> MIIKRTPQAASPLASWLSYLENLHSKTIDLGLERVSLVAARLGVLKPAPFVFTVAGTNGKGTTCRTLES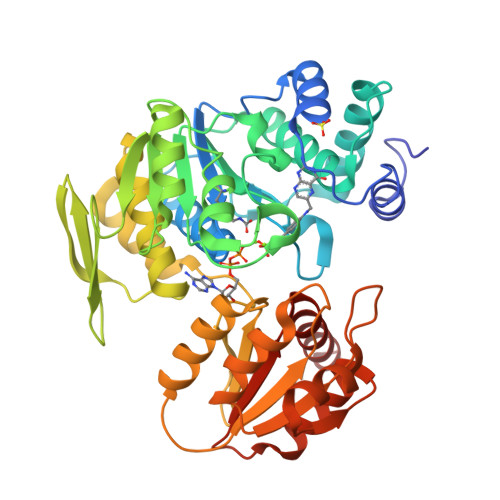ILMAAGYKVGVYSSPHLVRYTERVRVQGQELPESAHTASFAEIESARGDISLTYFEYGTLSALWLFKQAQLDVVILEVGLGGRLDATNIVDADVAVVTSIALDHTDWLGPDRESIGREKAGIFRSEKPAIVGEPEMPSTIADVAQEKGALLQRRGVEWNYSVTDHDWAFSDAHGTLENLPLPLVPQPNAATALAALRASGLEVSENAIRDGIASAILPGRFQIVSESPRVIFDVAHNPHAAEYLTGRMKALPKNGRVLAVIGMLHDKDIAGTLAWLKSVVDDWYCAPLEGPRGATAEQLLEHLGNGKSFDSVAQAWDAAMADAKAEDTVLVCGSFHTVAHVMEVIDARRSGGK[2'-HYDROXY-3'-(1H-PYRROLO[3,2-C]PYRIDIN-2-YL)-BIPHENYL-3-YLMETHYL]-UREA | 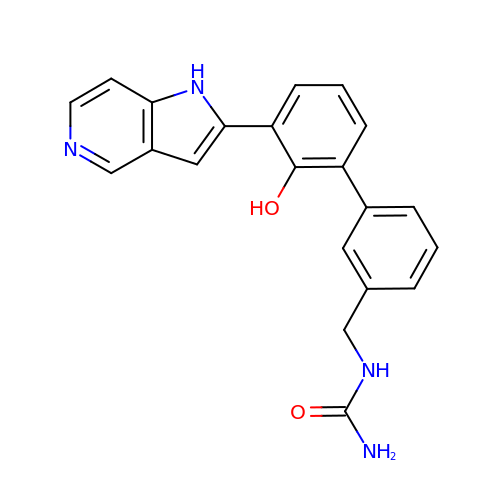C21 H18 N4 O2 | SRPOHNDQBDHONJ-UHFFFAOYSA-N>GSMHWNDLLNSNRRKPKNEKKESSQDTSKGRQQIERDYDRILFAAPTRRLADKTQVFPLDKNDSVRTRLTHSHEVANLSRGIGMRLAFELEDDVFKDVSEDICLKRDVPALLAAIGLVHDMGNPPFGAQGAKAMSEWFTKNLPEHSDNYKDKIYGDFRHFDGNSQTLRLVTKLQILNDTYGLNLTYATLASMIKYPRSSESDSSLWKKHGFFLSEKDVVQDIWNNTGLSEGVRHPFTYIMEACDDIAYSVLDAEDIIKKGFASFHDLIDFIQSNQFCKEDDVAKRVIENCKKIHADYAQQKLSPAELNDMSMQMFRVYAIAELVDAVVIAFKDNINEFLNDTCEIKDLISCSSGKNLCQALKKFDSSRGYQHRSVLKLELEGSNYIKGLMDMLWLGIKGRATGDTQYDTPFGRYVYGRISENYRRIFEQENNLPACYKEAQLLADAISGMTDSYLIALHDELRALHQYECR[8x]

pmcDeoxynucleoside triphosphohydrolase (dNTPase) enzymes are effector proteins in animal and bacterial cells that hydrolyze dNTP nucleotides and inhibit viral replication. We therefore named the dNTPase-NTase anti-phage defense system Clover and designated the dNTPase protein as Clover protein A (CloA) and the accessory NTase protein as Clover protein B (CloB). Likewise, CloA exhibits strict dGTP substrate specificity, with the activated enzyme only hydrolyzing dGTP and leaving other dNTPs including dTTP unaffected. Together these results demonstrate that CloA is a dGTPase effector that senses phage infection by specifically responding to elevated dTTP concentrations associated with viral replication. Clover defense encodes an accessory enzyme CloB that synthesizes an additional nucleotide signal p3diT that suppresses CloA activation and protects uninfected cells from aberrant nucleotide depletion. p3diT binds to CloA in an allosteric site adjacent to the dTTP binding pocket and raises the threshold of intracellular dNTP levels required to trigger full Clover immune activation.

To define the mechanism of nucleotide signaling in Clover anti-phage defense, we mutated the Salmonella CloA active site (H126A/E129A) to allow direct comparison of dGTP substrate interactions and determined cryo-EM structures of CloA in the suppressed CloA–dGTP–p3diT (2.6 Å) or activated CloA–dGTP–dTTP (2.6 Å) states. Remarkably, the CloA–dGTP–p3diT and CloA–dGTP–dTTP structures reveal that p3diT and dTTP each bind at the CloAAB interface in structurally distinct sites that remodel to accommodate the inhibiting or activating nucleotide signals. In the CloA–dGTP–dTTP active state structure, dTTP is bound at the CloAAB interface in an adjacent pocket to the p3diT binding site formed by loops α3A–α4A and α3B–α4B from each CloA protomer and the C-terminal helical bundle α18B–α21B. A distinct set of conserved CloA residues form 13 hydrogen-bond interactions with dTTP that coordinate the nucleotide triphosphate moiety at each of the α-(R47A and S418A), β- (K256B), and γ-phosphate (R47A, Q172A, and N420A) positions. The dTTP ribose sugar backbone is coordinated by the side-chain of CloA residue R47A and the peptide main-chain of residue A444A. The thymidine base is recognized by an extensive series of interactions with CloA residues R47A and Y452A that sandwich the nucleobase face and residues D61B and T449A that make sequence-specific contacts along the Watson-Crick edge and explain the exquisite specificity of CloA for dTTP as an activating nucleotide signal. In contrast, in the dTTP-bound active state, dGTP is coordinated by an additional set of five contacts that reorient substrate interactions and complete active site formation. First, dTTP-binding induces a conformational change that repositions sidechain R66A to form new hydrogen bond interactions with the peptide backbone of T52A, Q53A, and N121A that stabilize loop α3A–α4A in the dGTPase core.>MQDITMQWYQQLQDASMQCVLTFEGLTNSKDSQAKKIKMDLQKAATIPVSQISTIAGSKLKEIFDKIHSLLSGKPVQSGGRSVSVTLNPQGLDFVQYKLAEKFVKQGEEEVASHHEAAFPIAVVASGIWELHPRVGDLILAHLHKKCPYSVPFYPTFKEGMALEDYQRMLGYQVKDSKVEQQDNFLKRMSGMIRLYAAIIQLRWPYGNRQEIHPHGLNHGWRWLAQILNMEPLSDVTATLLFDFLEVCGNALMKQYQVQFWKMLILIKEDYFPRIEAITSSGQMGSFIRLKQFLEKCLQHKDIPVPKGFLTSSFWRS[2x];>GPSGSIIATDNVLFTPRDKLTVEELEQFQSKKFTLGKIPLKPPPLELLNV[2x]

At the cytoplasmic face of the NPC, Nxf1•Nxt1-bound mRNPs encounter the cytoplasmic filament nucleoporins Gle1, Nup42, and Nup214, which specifically activate the DEAD-box helicase DDX19 to remove Nxf1•Nxt1 from the mRNP8. DDX19 is a member of the DEAD-box helicase family, which are RNA-dependent ATPases composed of two RecA domains (referred to as DDX19NTD and DDX19CTD throughout the text). Gle1CTD plays an important organizational role by providing spatially separated binding sites for Nup42GBM and the DEAD-box helicase DDX19/scDbp5. A comprehensive structure-function analysis of DDX19 indicates that binding of Gle1CTD•Nup42GBM induces a conformational change in DDX19, thereby stimulating its ATPase activity.

The difficulty of purifying human Gle1CTD has previously prevented a detailed biochemical analysis of the human proteins, but the dramatic effect of yeast Nup42GBM on Gle1CTD stability led us to test whether human Nup42GBM has the same effect on human Gle1CTD. Co-purification of a homologous human Gle1CTD•Nup42GBM complex (containing Gle1 residues 382−698 and Nup42 residues 379−423) resulted in dramatic improvements in the stability of Gle1CTD and the yields increased from ~0.5 to ~50 mg/100 l of bacterial culture. In thermostability experiments, the Tm of human Gle1CTD increased from 37 to 50 °C in the presence of Nup42GBM. To evaluate whether the mode of interaction observed for S. cerevisiae Gle1CTD•Nup42GBM was conserved in other eukaryotes, we determined the crystal structures of human Gle1CTD•Nup42GBM at 2.8 Å resolution and of C. thermophilum Gle1CTD•Nup42GBM in the presence and absence of IP6 at 2.17 and 2.65 Å resolution, respectively. The overall structure of Gle1CTD is conserved between fungi and humans, with minor differences resulting from small insertions or different loop sizes. Both human and C. thermophilum Nup42GBM adopt the same fold as S. cerevisiae Nup42GBM and recognize the same surface on Gle1CTD, with the critical hydrophobic residues nearly universally conserved. However, no binding of IP6 to human Gle1CTD•Nup42GBM was detected up to concentrations of 200 μM. All three LCCS1/LAAHD mutations possessed altered thermostability that correlated with their phenotypic disease manifestation, with the R569H variant exhibiting the largest difference in Tm, from 50 °C for wild-type protein to 40 °C for the disease variant. In our crystal structures, R569 is involved in an extensive network of intra-molecular interactions, whereas V617 and I684 are both buried in hydrophobic cores, supporting the conclusion that these mutations reduce the stability of Gle1 rather than affecting their ability to stimulate the activity of DDX19.> MSRLDK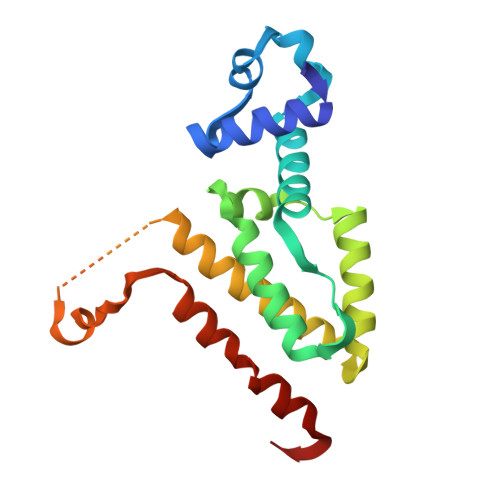SKVINSALELLNEVGIEGLTTRKLAQKLGVEQPTLYWHVKNKRALLDALAVEILARHHDYSLPAAGESWQSFLRNNAMSFRRALLRYRDGAKVHLGTRPDEKQYDTVETQLRFMTENGFSLRDGLYAISWVSHFTLGAVLEQQEHTAALTDRPAAPDENLPPLLREALQIMDSDDGEQAFLHGLESAIRGIEVQLTALLQIV> MNYWWVSQKQTFKQEFEGGYMWSPKENKNGTQSHYYNNMTLVQPGDVVFSFANGLILSVGIARSHAYSYNKPTEFGVAGADWANDGWKIDLEYHLVENKIRPKAHIDFIRPYLPQKYSPLQDNGNGNQAYLFSVPHELASKV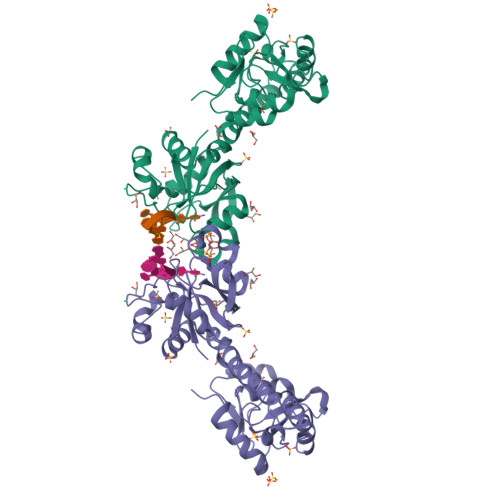VELIGSEAEEVIFGFADTTEITTTADAIECQISNDASIDETEKHQLVKSRRGQGIFRSRLEQVESRCRVTGVQLKNHLIASHIKPWAVSNNQERLDGHNGLLLAPHVDHLFDKGFISFEDNGEMIVSEKLNLDVLKAWSISQGNYGYFSKQQQEYMCYHRENVFKKL>[4x]GMDKYLSANSLEGVIDNEFSMPAPRWLNTYPAGP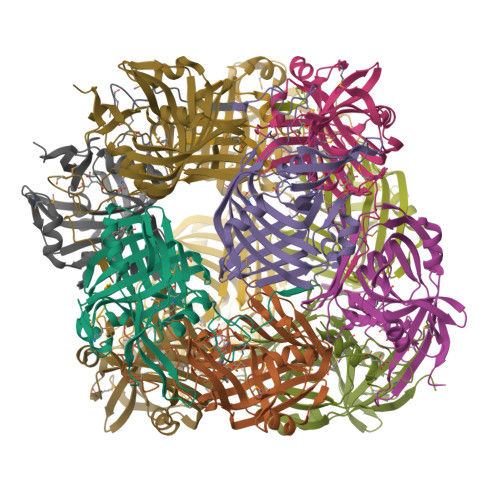YRFINREFFIIAYETDPDLLQAILPPDMELLEPVVKFEFIRMPDSTGFGDYTESGQVVPVRYKGEEGGFTISMFLDCHAPIAGGREIWGFPKKLAKPKLFVEEDTLIGILKYGSIDIAIATMGYKHRPLDAEKVLESVKKPVFLLKNIPNVDGTPLVNQLTKTYLTDITVKGAWTGPGSLELHPHALAPISNLYIKKIVSVSHFITDLTLPYGKVVADYLA> MQDNSRYTHFLTQHYDAKPQGRDDRYCESIMRRRGLTSPCRDINTFIHGNKRSIKAICENKNGNPHRENLRI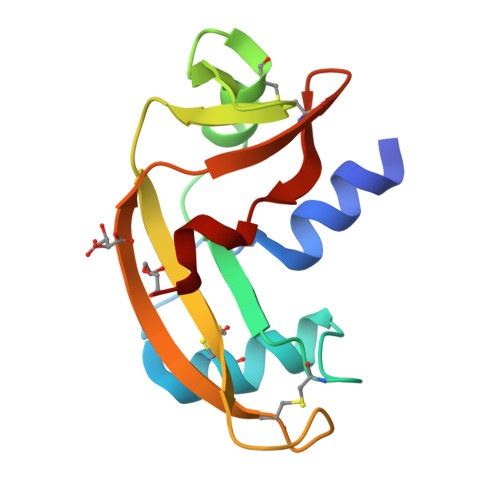SKSSFQVTTCKLHGGSPWPPCQYRATAGFRNVVVACENGLPVHLDQSIFRRP>KEATWVTDKPLTLKIHMHFRDKWVWDENWPVAKESFRLTNVKLQSVANKAATNSQEQFNLMMASGDLPDVVGGDNLKDKFIQYGQEGAFVPLNKLIDQYAPHIKAFFKSHPEVERAIKAPDGNIYFIPYVPDGVVARGYFIREDWLKKLNLKPPQNIDELYTVLKAFKEKDPNGNGKAAAVPFIDRHPDEVFRLVNFWGARSSGSDNYMDFYIDNGRVKHPWAETAFRDGMKHVAQWYKEGLIDKEIFTRKARAREQMFGGNLGGFTHDWFASTMTFNEGLAKTVPGFKLIPIAPPTNSKGQRWEEDSRQKVRPDGWAITVKNKNPVETIKFFDFYFSRPGRDISNFGVPGVTYDIKNGKAVFKDSVLKSPQPVNNQLYDMGAQIPIGFWQDYDYERQWTTPEAQAGIDMYVKGKYVMPGFEGVNMTREERAIYDKYWADVRTYMYEMGQAWVMGTKDVDKTWDEYQRQLKLRGLYQVLQMMQQA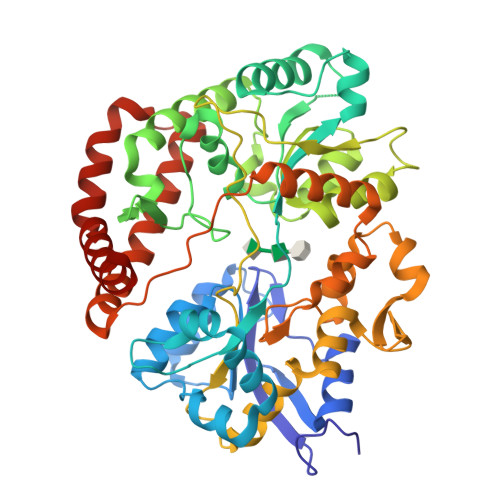YDRQYKN[2x]> MELFDENYYAKAVANIIGEVKDPIMYKWFSPDQIEDVDLQMGYQKTVKWDAFLNANPTTIANEVNTISTIGFSSEVVRLNYLKLQYKFRHLKQTSEKFYTSDSYIGDINNNLLPFAQAYKLASSEIIK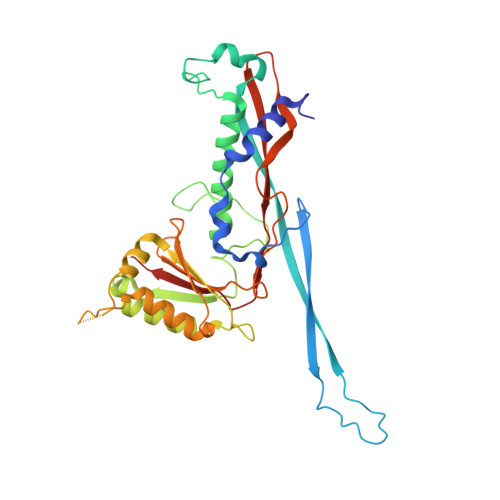LINHFVLTGTVSIQKDGKNQKRLLPNMYGLLNMPEQIKEEVASGDKDKMDKIFEKIEAGLSKLELGDEFSTPMMVIVDPATSLKLVKPYAAAQGAASSCEKWEDVLIQTIKAINNREDVYIETSNLLKHKILIYPLNSELIKFKPSKYMLPTPNEQVDKDSTDVAHSYIDFVLGGLLATRKTILQVNIKQS> SRKTYTLTDYLKNTYRLKLYSLRWISDHEYLYKQENNILVFNAEYGNSSVFLENSTFDEFGHSINDYSISPDGQFILLEYNYVKQWRHSYTASYDIYDLNKRQLITEERIPNNTQWVTWSPVGHKLAYVWNNDIYVKIEPNLPSYRITWTGKEDIIYNGITDWVYEEEVFSAYSALWWSPNGTFLAYAQFNDTEVPLIEYSFYSDESLQYPKTVRVPYPKAGAVNPTVKFFVVNTDSLSSVTNATSIQITAPASMLIGDHYLCDVTWATQERISLQWLRRIQNYSVMDICDYDESSGRWNCLVARQHIEMSTTGWVGRFRPSEPHFTLDGNSFYKIISNEEGYRHICYFQIDKKDCTFITKGTWEVIGIEALTSDYLYYISNEYKGMPGGRNLYKIQLSDYTKVTCLSCELNPERCQYYSVSFSKEAKYYQLRCSGPGLPLYTLHSSVNDKGLRVLED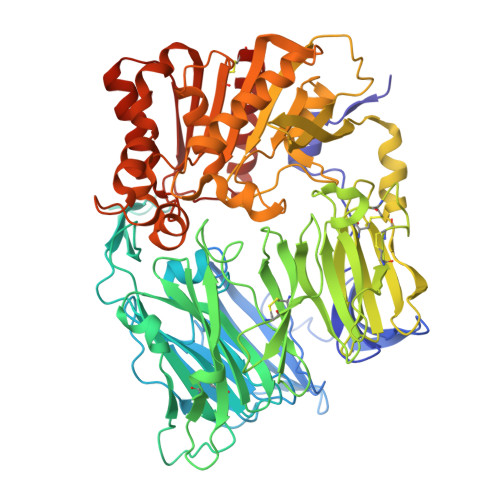NSALDKMLQNVQMPSKKLDFIILNETKFWYQMILPPHFDKSKKYPLLLDVYAGPCSQKADTVFRLNWATYLASTENIIVASFDGRGSGYQGDKIMHAINRRLGTFEVEDQIEAARQFSKMGFVDNKRIAIWGWSYGGYVTSMVLGSGSGVFKCGIAVAPVSRWEYYDSVYTERYMGLPTPEDNLDHYRNSTVMSRAENFKQVEYLLIHGTADDNVHFQQSAQISKALVDVGVDFQAMWYTDEDHGIASSTAHQHIYTHMSHFIKQCFSLP> MLKQVEIFTDGSALGNPG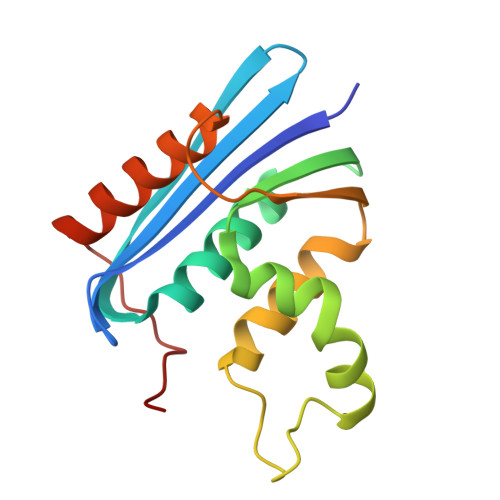PGGYGAILRYRGREKTFSAGYTRTTNNRMELMAAIVALEALKEHAEVILSTDSQYVRQGITQWIHNWKKRGWKTADKKPVKNVDLWQRLDAALGQHQIKWEWVKGHAGHPENERADELARAAAMNPTLEDTGYQVEV>[2x]MSAPRGDHAILRARNLTKRVATLGPSTDVLRPDELIKFLDLVDGVRINLAHASPNEVKFRIEAVRSYEKAKNRPLAVIVDLKGPSIRV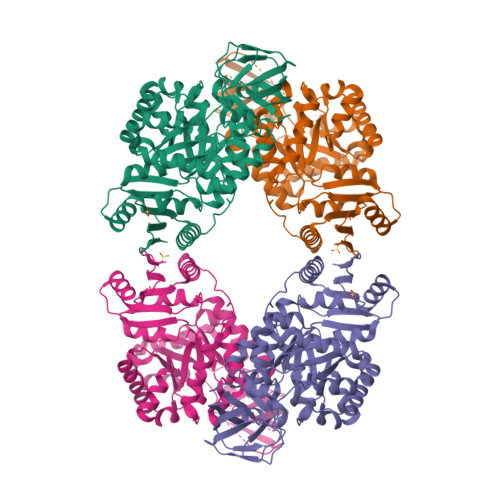GSTSPINVQEGEVVKFKLSDKSDGTYIPVPNKAFFSAVEQNDVILMLDGRLRLKVTNTGSDWIEAVAESSGVITGGKAIVVEGKDYDISTPAEEDVEALKAISPIRDNIDYVAISLAKSCKDVDSVRSLLTELGFQSQVAVKIETKGAVNNLEELVQCSDYVVVARGDLGLHYGLDALPIVQRRIVHTSLKYGKPIAVATQLLDSMQSSPIPTRAEINDVFTTASMGVDSLWLTNETASGKYPLAAVSWLSRILMNVEYQIPQSPLLQNSRDRFAKGLVELAQDLGANILVFSMSGTLARRIAKFRPRGVVYVGTPNVRVARSLSIVWALEPLYIPAENYEEGLEKLISLKGTTPFVATYGIRGGVHSVKVKL During activation of a pentameric ligand-gated ion channel (pLGIC), the binding of agonists promotes the opening of a selective ion conduction pore at a distance of more than 50 Å away from the binding sites. Each subunit consists of a predominantly β-stranded extracellular domain and an α-helical transmembrane pore, which interact via an extended interface. Whereas ELIC forms a cation-selective channel with high conductance that is activated with high efficacy by the primary amines cysteamine, propylamine, and GABA, the cation-selective GLIC is activated by protons and inhibited by bulky positively charged compounds that also act as open channel blockers of the nAChR. Our study has identified a cluster of interacting residues located at the β1-β2 turn, the β6-β7 loop and the pre-M1 region of the extracellular domain, and the M2-M3 loop of the pore that exert a strong influence on channel function.

For two cases, the ELIC mutants F116A of the β6-β7 loop and Y258A of the M2-M3 loop, we have grown crystals and determined structures at 3.5 and 3.2 Å, respectively. Both mutants crystallized in the same nonconducting conformation that has been observed in all known ELIC structures. Small structural differences in the vicinity of the respective mutations indicate local rearrangements of protein interactions due to the loss of the bulky aromatic side chains. The data suggests that the mutations, despite their severe phenotype on channel activation, have only a local effect on the protein structure. We have also investigated whether both mutants would at least show residual activity, and we have thus expressed them in X. laevis oocytes and HEK-293 cells and studied excised patches in the outside-out configuration upon fast application of agonist. Neither of the two mutants display ligand-induced channel activity in any of numerous independent recordings. To exclude that the two nonactivating mutations have compromised the ability of the protein to recognize its ligand, we have studied agonist and antagonist binding to the detergent solubilized protein by isothermal titration calorimetry (ITC). In the background of the mutant R91A, both nonactivatable mutants F116A and Y258A bind agonist and antagonist with similar Keff as the single mutant R91A, thus emphasizing that the mutation has likely not affected ligand binding but instead interfered with channel activation. In both nonconducting conformations, the interactions with the C-terminal part of the M2-M3 loop with the β6-β7 linker remain intact, and the observed nonactivating phenotype of respective mutations (F116A and Y258A in ELIC and F115A and Y250A in GLIC) could thus originate from an interruption of the coupling between the extracellular domain and the pore region.

>[10x]APADNAADARPVDVSVSIFINKIYGVNTLEQTYKVDGYIVAQWTGKPRKTPGDKPLIVENTQIERWINNGLWVPALEFINVVGSPDTGNKRLMLFPDGRVIYNARFLGSFSNDMDARLFPFDRQQFVLELEPFSYNNQQLRFSDIQVYTENIDNEEIDEWWIRGKASTHISDIRYDHLSSVQPNQNEFSRITVRIDAVRNPSYYLWSFILPLGLIIAASWSVFWLESFSERLQTSFTLMLTVVAYAFYTSNILPRLPYTTVIDQMIIAGYGSIFAAILLIIFAHHRQANGVEDDLLIQRCRLAFPLGFLAIGCVLVIRGITL>[4x]MNKGELVDAVAEKASVTKKQADAVLTAALETIIEAVSSGDKVTLVGFGSFESR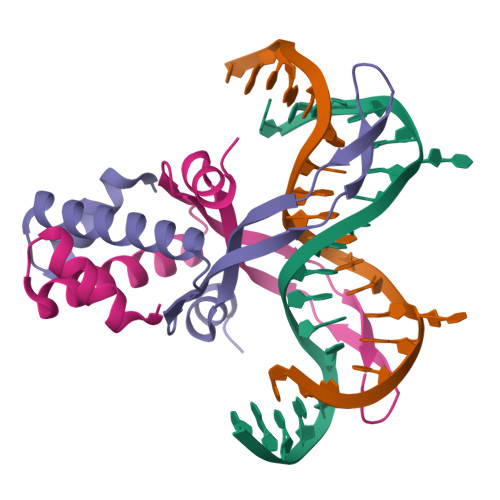ERKAREGRNPKTNEKMEIPATRVPAFSAGKLFREKVAPPKA> ANVRLQHHHHHHHLEGSFIDNSSVELTTRNFYFDRDYQEQSAYPAAKDWTQGFILKANSGYTEGTIGFGLDVLATAGFKLDADAEHGG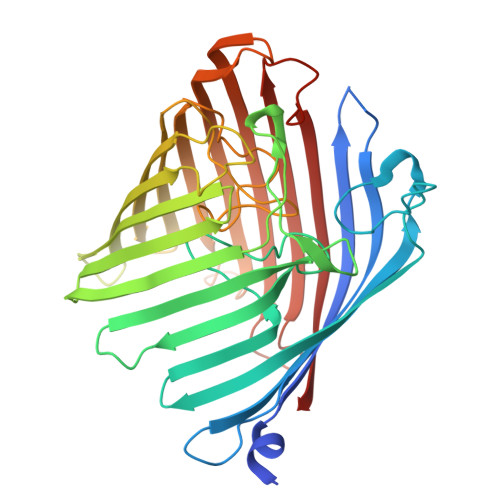TGNLPRDTRTNEPADSYGEIGVTAKAKMSQTELRIGTLMPMNPVLVASPARLLPQTYRGISLTSKDIKDFDLQAAYLDKVNHRDSTNYEKIKISGVNGRFKGAETDGLYYLGGNYQFNPALKLTAFYMDVDDLYNQTMVGALHQYKINDTTNFSSQLRYYRSRDDGQAKAGLVDNDLYHAHFELKHQNHKFIFGTFQHHGDTAFPYLTGGETGLLIDTWPGEFLNPKEKAYSFRYEYDFKEYVPGLCFMTRYTTGHNIYAPNLGGTNLKERETDFDLGYTVQSGWLKNLGLRARYAIYDNNMLSTANIKPVNETRINIDYTWKFK> SQIPASEQ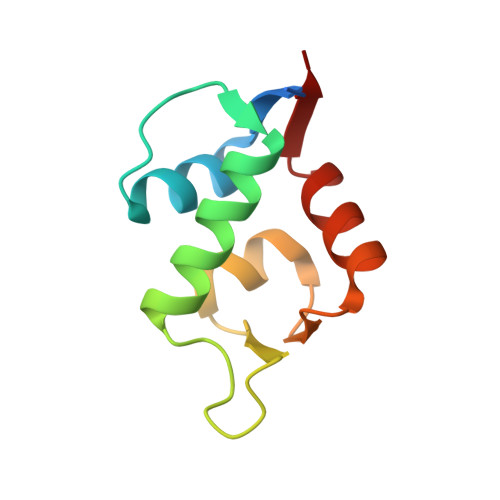ETLVRPKPLLLKLLKSVGAQKDTYTMKEVLFYLGQYIMTKRLYDEKQQHIVYCSNDLLGDLFGVPSFSVKEHRKIYTMIYRNLVVVN> MASNEGVENRPFPYLTVDADLLSNLRQSAAEGLFHSFDLLVGKDAREAGIKFEVLLGVYTNAIQYVRFLETALAVSCVNTEFKDLSRMIDGKIQFRISVPTIAHGDGRRPSKQRTFIVVKNCHKHHISTEMELSMLDLEILHSIPETPVEYAEYVGAVKTVASALQFGVDALERGLINTVLSVKLRHAPPMFILQTLADPTFTERGFSKTVKSDLIAMFKRHLLEHSFFLDRAENMGSGFSQYVRSRLSEMVAAVSGESVLKGVSTYTTAKGGEPVGGVFIVTDNVLRQLLTFLGEEADNQIMGPSSYASFVVRGENLVTAVSYGRVMRTFEHFMARIVDSPEKAGSTKSDLPAVAAGVEDQPRVPISAAVIKLGNHAVAVESLQKMYNDTQSPYPLNRRMQYSYYFPVGLFMPNPKYTTSAAIKMLDNPTQQLPVEAWIVNKNNLLLAFNLQNALKVLCHPRLHTPAHTLNSLNAAPAPRDRRETYSLQHRRPNHMNVLVIVDEFYDNKYAAPVTDIALKCGLPTEDFLHPSNYDLLRLELHPLYDIYIGRDAGERARHRAVHRLMVGNLPTPLAPAAFQEARGQQFETATSLAHVVDQAVIETVQDTAYDTAYPAFFYVVEAMIHGFEEKFVMNVPLVSLCINTYWERSGRLAFVNSFSMIKFICRHLGNNAISKEAYSMYRKIYGELIALEQALMRLAGSDVVGDESVGQYVCALLDPNLLPPVAYTDIFTHLLTVSDRAPQIIIGNEVYADTLAAPQFIERVGNMDEMAAQFVALYGYRVNGDHDHDFRLHLGPYVDEGHADVLEKIFYYVFLPTCTNAHMCGLGVDFQHVAQTLAYNGPAFSHHFTRDEDILDNLENGTLRDLLEISDLRPTVGMIRDLSASFMTCPTFTRAVRVSVDNDVTQQLAPNPADKRTEQTVLVNGLVAFAFSERTRAVTQCLFHAIPFHMFYGDPRVAATMHQDVATFVMRNPQQRAVEAFNRPEQLFAEYREWHRSPMGKYAAECLPSLVSISGMTAMHIKMSPMAYIAQAKLKIHPGVAMTVVRTDEILSENILFSSRASTSMFIGTPNVSRREARVDAVTFEVHHEMASIDTGLSYSSTMTP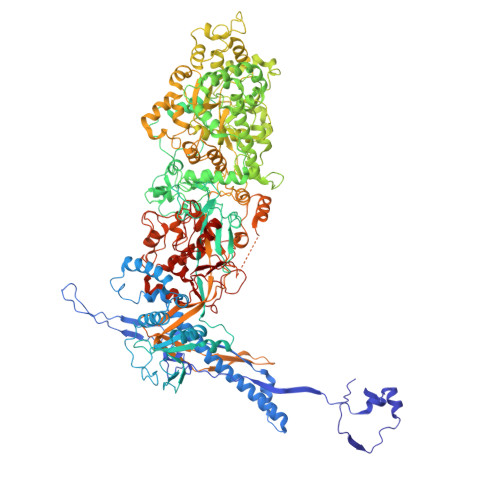ARVAAITTDMGIHTQDFFSVFPAEAFGNQQVNDYIKAKVGAQRNGTLLRDPRTYLAGMTNVNGAPGLCHGQQATCEIIVTPVTADVAYFQKSNSPRGRAACVVSCENYNQEVAEGLIYDHSRPDAAYEYRSTVNPWASQLGSLGDIMYNSSYRQTAVPGLYSPCRAFFNKEELLRNNRGLYNMVNEYSQRLGGHPATSNTEVQFVVIAGTDVFLEQPCSFLQEAFPALSASSRALIDEFMSVKQTHAPIHYGHYIIEEVAPVRRILKFGNKVVF>YTKFAPPGKPSLGWGERTFAIVEVNQAATAYNQLVTKRDSADVSVTWNVWSGDPADKARVLLNDKEFWSGTGGAAGSASFKVKKGGRYQMVVELCNADGCSQSDATEIIVADTDGSHLPPLDYNMGEKNKPFKQTSGKVVGAYFVEWGVYPRKFPVDRVPIPNLTHLLYGFIPICGGDGINDSLKEIEGSFQALQRSCSGREDFKVSIHDPWAALQKPQKGLSSWNEPYKGNFGQLMMLKQAKPDLKILPSIGGWTLADPFFFFT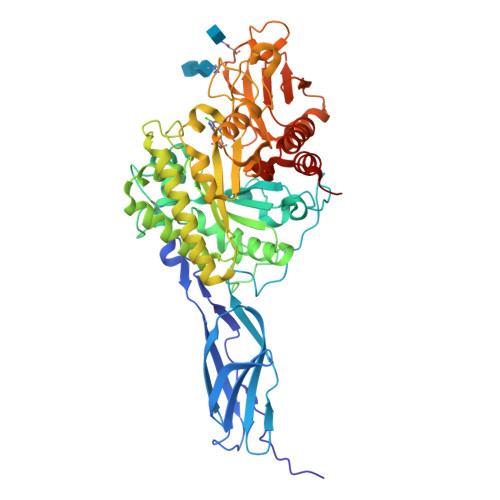DETKRRRFVASVKDFLQTWKFFDGVDIDWEFPGGKGANPNLGSPKDGEIYVLLMKELREMLNELSAETGRKYELTSAISAGWDKIQVVDYSAAQKYMDHIFFMSYDFKGAWSNDTLGHQASLYAPDWNEKETYTTDFGVQFLLAQGVSPKKIVVGVAMYGRGWTGVHGYKDNNPFTGNATGPVKGTWQDGVVDYREIATEIAQGKWEYHYDKVAQAPYVFRPATGDLITYDDARSTIEKGKYVRANKLGGLFAWEIDADNGDILNAMNMGLGNSA[2x]>DLLAGGKDDVKATFGADSFVMMCIIIAELIVGVAMYIRTKNLLILLGLVVVIVFTTVGLTFIK[80x]

Conjugative pili are widespread bacterial appendages that play important roles in horizontal gene transfer, in spread of antibiotic resistance genes, and as sites of phage attachment. The pilus is a polymer of the VirB2 protein (or pilin). The structures of the pED208 and F pilus are very similar, with overall dimensions of 87 Å in diameter and an internal lumen of 28 Å in diameter. Thus, selective binding of PG to pilins occurs in both F and pED208 pili, and thus, the F family of pili are polymers of a selective and stoichiometric protein-PG complex unit.

For pED208, a 3.6 Å resolution map was generated in which α-helical secondary structures, as well as most side chains, were clearly visible and in which a model for the pED208 pilin, TraA, could be readily built and refined with excellent stereochemistry. During the process of helical reconstruction, as the resolution was increased, an additional separate density became clearly visible and readily interpretable as a phospholipid. For pED208, the angle between adjacent subunits is 28.2° and the rise is 12.1 Å, while for the two F pilus structures, the helical parameters were 27.9° with a rise of 13.2 Å and 28.1° with a rise of 12.5 Å, respectively. The pED208 TraA pilin is a 64-residue protein, 63 of which (residues 2–64) were clearly defined in the electron density. TraA folds into an all-α-helical structure, containing three α helices (α1–3). TraA orientation within the pilus is such that the loop between α2 and α3 is located within the lumen of the pilus, while the N- and C-terminal ends are located on the outside of the filament. As resolution increased, clear density resolved the head group and acyl chains of a phospholipid stoichiometrically interacting with the pilin. Two main species bound to the pilin were identified by daughter ion fragmentation as phosphatidylglycerol (PG) species, PG 32:1(16:0, 16:1) and PG 34:1 (16:0, 18:1). Each lipid molecule makes extensive contacts with five surrounding TraA subunits, while each TraA subunit interacts with five lipid molecules. In the lipid, only the head groups are solvent exposed and directed to the lumen of the pilus.>MAMITGGELVVRTLIKAGVEHLFGLHGSHIDTIFQACLDHDVPIIDTRHEAAAGHAAEGYARAGAKLGVALVTAGGGFTNAVTPIANAWLDRTPVLFLTGSGALRDDETNTLQAGIDQVAMAAPITKWAHRVMATEHIPRLVMQAIRAALSAPRGPVLLDLPWDILMNQIDEDSVIIPDLVLSAHGARPDPADLDQALALLRKAERPVIVLGSEASRTAR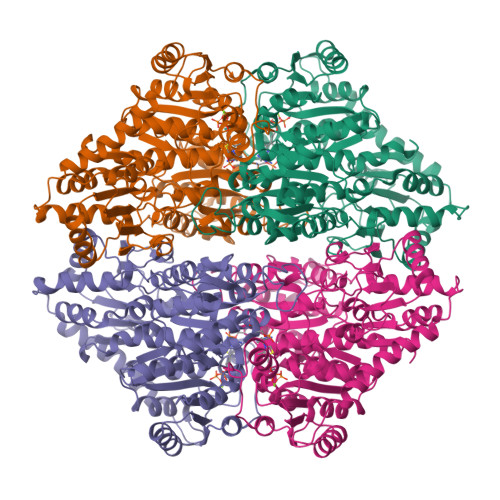KTALSAFVAATGVPVFADYEGLSMLSGLPDAMRGGLVQNLYSFAKADAAPDLVLMLGARFGLNTGHGSGQLIPHSAQVIQVDPDACELGRLQGIALGIVADVGGTIEALAQATAQDAAWPDRGDWCAKVTDLAQERYASIAAKSSSEHALHPFHASQVIAKHVDAGVTVVADGALTYLWLSEVMSRVKPGGFLCHGYLGSMGVGFGTALGAQVADLEAGRRTILVTGDGSVGYSIGEFDTLVRKQLPLIVIIMNNQSWGATLHFQQLAVGPNRVTGTRLENGSYHGVAAAFGADGYHVDSVESFSAALAQALAHNRPACINVAVALDPIPPEELILIGMDPFGSHHHHHH[4x]> GPAVQDVVDQFFQPVKPTLGQIVRQKLSEGRKVTCRLLGVILEETSPEELQKQATVRSSVLEVLLEITKYSDLYLMERVLDDESEAKVLQALENAGVFTSGGLVKDKVLFCSTEIGRTSFVRQLEPDW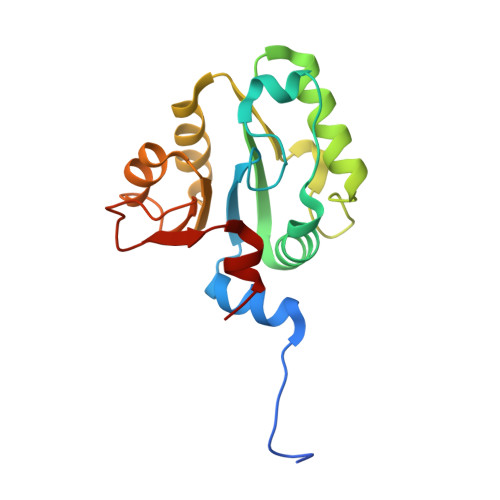HIDTNPEISTQLARFIKYQLHVATVKPERTAPNVFTSQSIEQFFGSV>[2x]MSVGRRRIKLLGILMMANVFIYFIMEV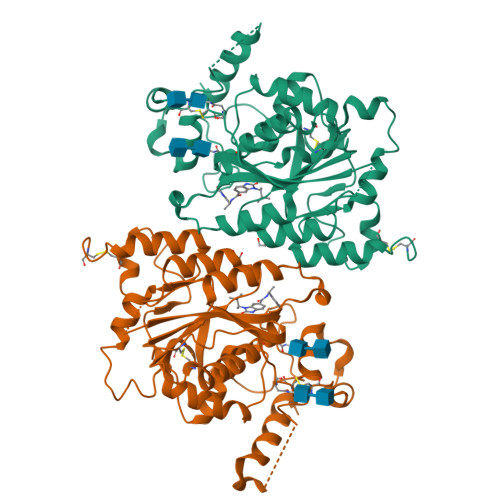SKSSSQEKNGKGEVIIPKEKFWKISTPPEAYWNREQEKLNRQYNPILSMLTNQTGEAGRLSNISHLNYCEPDLRVTSVVTGFNNLPDRFKDFLLYLRCRNYSLLIDQPDKCAKKPFLLLAIKSLTPHFARRQAIRESWGQESNAGNQTVVRVFLLGQTPPEDNHPDLSDMLKFESEKHQDILMWNYRDTFFNLSLKEVLFLRWVSTSCPDTEFVFKGDDDVFVNTHHILNYLNSLSKTKAKDLFIGDVIHNAGPHRDKKLKYYIPEVVYSGLYPPYAGGGGFLYSGHLALRLYHITDQVHLYPIDDVYTGMCLQKLGLVPEKHKGFRTFDIEEKNKNNICSYVDLMLVHSRKPQEMIDIWSQLQSAHLKC>[2x]VLDSFEILKALKSLDLLKNAPAW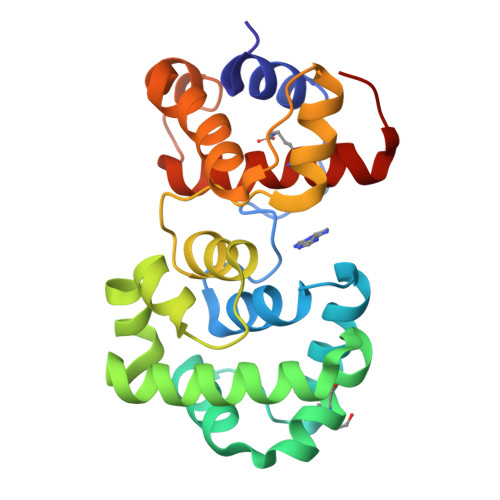WWPNALKFEALLGAVLTQNTKFEAVLKSLENLKNAFILENDDEINLKKIAYIEFSKLAECVRPSGFYNQKAKRLIDLSGNILKDFQSFENFKQEVTREWLLDQKGIGKESADAILCYACAKEVMVVDKYSYLFLKKLGIEIEDYDELQHFFEKGVQENLNSALALYENTISLAQLYARFHGKIVEFSKQKLELKL> MPDIKITPLGAGQDVGRSCLLLSMGGKNIMLDCGMHMGYNDERRF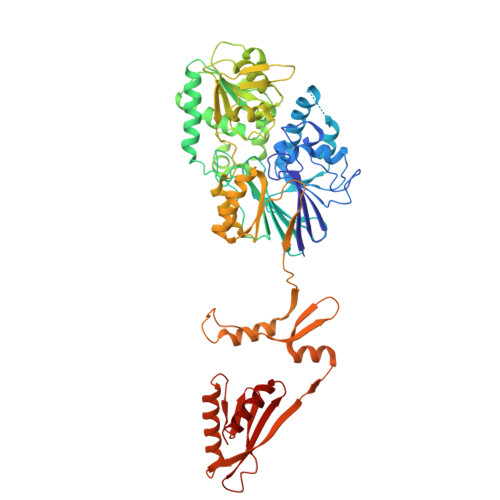PDFSYIVPEGPITSHIDCVIISHFHLDHCGALPYMSEIVGYTGPIYMTHPTKAIAPILLEDMRKVAVERKGESNFFTTQMIKDCMKKVIPVTLHQSMMVDTDLEIKAYYAGHVLGAAMFWIKVGSQSVVYTGDYNMTPDRHLGAAWIDKCRPDLLISESTYATTIRDSKRCRERDFLKKVHECVAKGGKVLIPVFALGRAQELCILLETYWERMNLKYPIYFALGLTEKANTYYKMFITWTNQKIRKTFVHRNMFDFKHIKPFDKAYIDNPGAMVVFATPGMLHAGLSLQIFKKWAPNENNMVIMPGYCVQGTVGNKILGGAKKVEFENRQVVEVKMAVEYMSFSAHADAKGIMQLIQNCEPKNVMLVHGEAGKMKFLRSKIKDEFNLETYMPANGETCVISTPVKIPVDASVSLLKAEARSYNAQPPDPKRRRLIHGVLVMKDNRIMLQNLTDALKEIGINRHVMRFTSKVKMDDSGPVIRTSERLKTLLEEKLAGWTVTMQENGSIAIESVEVKVEEDEKDPKQKNILISWTNQDEDIGAYILNVLQNMC>MLEETEAALLARVRELFGATLRQVEPLTGTWTNEDVHRLFLAPPSVFLAWMGCGEGRTRREVESRWAFFVVAELLNGEPVNRPGIYQIVERLIAGVNGQTFGPTTGMRLTQVRNLCDDNRINAGVVLYGVLFSGTTPLPSVVDLDSLDDYERHWQTWKFPDETPEFAAHINVNQEKDHDAEN[6x];>MAGNQRQGVAFIRVNGMELESMEGASFTPSGITREEVTGSRVYGWKGKPRAAKVECKIPGGGPIGLDEIIDWENITVEFQADTGETWMLANAWQADEPKNDGGEISLVLMAKQSKRIA[12x];>[12x]MSDISFNAIPSDVRVPLTYIEFDNSNAVSGTPAPRQRVLMFGQSGSKASAAPNVPVRIRSGSQASAAFGQGSMLALMADAFLNANRVAELWCIPQGNGTGNAAVGEISLSGTAGENGSLVTYIAGQRLAVSVAAGATGAALADLLVARIKGQPDLPVTAEVRADSGDDDTHADVVLSAKFTGALSAVDVRWNYYAGETTPYGIITAFKAASGKNGNPDISASIAGMGDLQYKYIVMPYTDEPNLNLLRTELQERWGPVNQADGFAVTVLSGTYGDISTFGVSRNDHLISCMGIAGAPEPSYLYAATLCAVASQALSIDPARPLQTLTLPGRMPPAVGDRFTWSERNALLFDGIS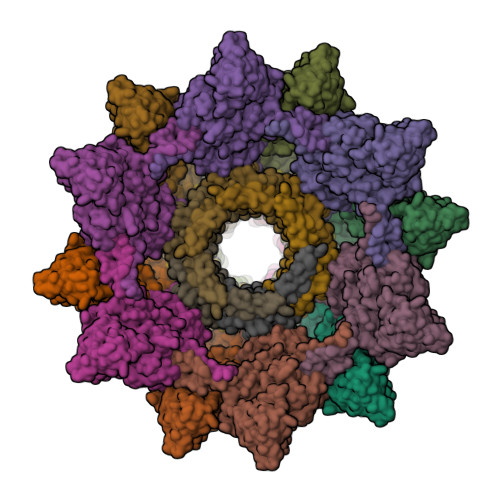TFNVNDGGEMQIERMITMYRTNKYGDSDPSYLNVNTIATLSYLRYSLRTRITQKFPNYKLASDGTRFATGQAVVTPSVIKTELLALFEEWENAGLVEDFDTFKEELYVARNKDDKDRLDVLCGPNLINQFRIFAAQVQFIL> MTFKAHVFDEPMLEFGDGGQHCDPRQGLREHGPLQPRSGDVIRVGVIGTDDTVAGFTEFLAETGRGIESGNKQLINLNPDFPGLGNQNPFRCKFEVPDGATVTISRRQVNDITGIGRHDEAVRHAVELISSQLSALVEGSAKPDVIVLALPIPLIEKLVNAKSEGEDSDDDVDGGDMLNFRDLLKAKTLHLPVPTQIVWPDTWDDAAKIPRKIKRDSNRQTQVKATRAWNLLNALFYKAGKVPWRLLPDQAEYRTSFLGIGFYRDLDGQQLWTSTAQMFDERGRGLILRGARAQTETRGRHPYLTAKDAEDLVVQ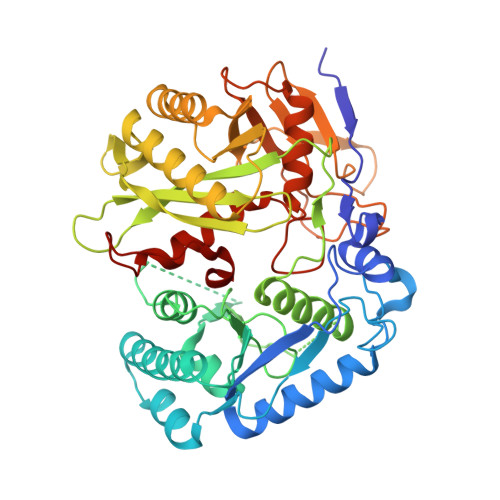SIAAYKAHHRHVPARLVVLKTSRFRSEEAEGIDAALGKSGIEMSDLVWVQESSPIAIFRDGNYPVLRGTFVDLDGKGLLYTRGSVPFYGTFPGLRVPRPLLLVPHENSDSTILTLAKDVLALTKVNWNTTQFDQKLPAPIKAAREVGRILKHVEFGTAVSSDFRRYT> SPLDQFEIRTLFGLQSSFIDLSCLNLTTFSLYTIIVLLVITSLYTLTNNNNKIIGSRWLISQEAIYDTIMNMTKGQIGGKNWGLYFPMIFTLFMFIFIANLISMIPYSFALSAHLVFIISLSIVIWL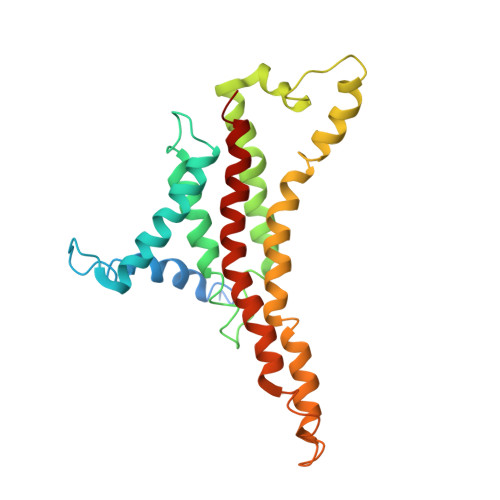GNTILGLYKHGWVFFSLFVPAGTPLPLVPLLVIIETLSYFARAISLGLRLGSNILAGHLLMVILAGLTFNFMLINLFTLVFGFVPLAMILAIMMLEFAIGIIQGYVWAILTASYLKDAVYLH> MAVTNEEIKTASKIVRRVSNVEAFDKSGSVFKGYQIWTDISPTIENDPNIMFVKCVVQQGSKKEKLTVVQIDPPGTGTPYDIDPTHAWNCNSQVDPMSFGDIGLLNHTNIPCVLDFLKHRYLKNQIYTTAVPLIVAINPYKDLGNTTNEWIRRYRDTADHTKLPPHVFTCAREALSNLHGVNKSQTIIVSGESGAGKTEATKQIMRYFASSKSGNMDLRIQTAIMAANPVLEAFGNAKTIRNNNSSRFGRFMQLVISHEGGIRYGSVVAFLLEKSRIITQDDNERSYHIFYQFLKGANSTMKSKFGLKGVTEYKLLNPNSTEVSGVDDVKDFEEVIESLKNMELSESDIEVIFSIVAGILTLGNVRLIEKQEAGLSDAAAIMDEDMGVFNKACELMYLDPELIKREILIKVTVAGGTKIEGRWNKNDAEVLKSSLCKAMYEKLFLWIIRHLNSRIEPEGGFKTFMGMLDIFGFEVFKNNSLEQLFINITNEMLQKNFVDIVFERESKLYKDEGISTAELKYTSNKEVINVLCEKGKSVLSYLEDQCLAPGGTDEKFVSSCATNLKENNKFTPAKVASNKNFIIQHTIGPIQYCAESFLLKNKDVLRGDLVEVIKDSPNPIVQQLFEGQVIEKGKIAKGSLIGSQFLNQLTSLMNLINSTEPHFIRCIKPNE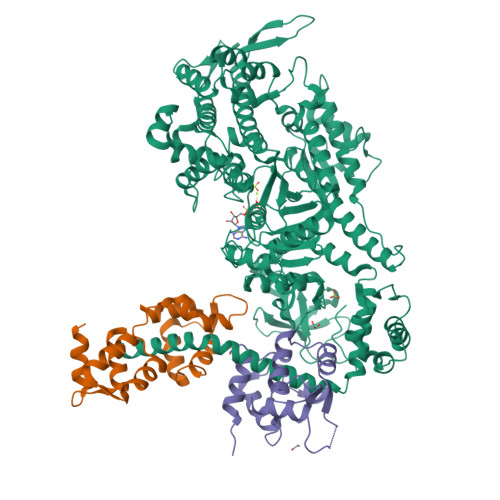NKKPLEWCEPKILIQLHALSILEALVLRQLGYSYRRTFEEFLYQYKFVDIAAAEDSSVENQNKCVNILKLSGLSESMYKIGKSMVFLKQEGAKILTKIQREKLVEWENCVSVIEAAILKHKYKQKVNKNIPSLLRVQAHIRKKMVAQ;> MKQECNVCYFNLPDPESTLGPYDNELNYFTWGPGFEYEPEPQRKPLSIEESFENSEESEESVADIQQLEEKVDESDVRIYFNEKSSGGKISIDNASYNARKLGLAPSSIDEKKIKELYGDNLTYEQYLEYLSICVHDKDNVEELIKMFAHFDNNCTGYLTKSQMKNILTTWGDALTDQEAIDALNAFSSEDNIDYKLFCEDILQ;> MASDMEEKFREAFILFSSCSDHIEMYKFFELMNSFGIILTNDEKAALPNDINMDYWLNFAKKHYNYEQPFKHINNVNEQNTNVQIKIDNFLGIMKALDTRLTESDLNILLQITNPENKSTLNLKTVSQKLTESI> GSDMRPEIWIAQEL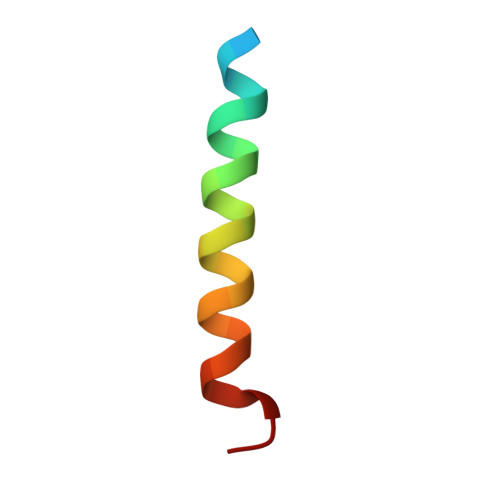RRIGDEFNAYYARR>MHHHHHHMELSLASITVPLESIKPSNILPVTVYDQHGFRILFHFARDPLPGRSDVLVVVVSMLSTAPQPIRNIVFQSAVPKVMKVKLQPPSGMELPAFNPIVHPSAITQVLLLANPQKEKVRLRYKLTF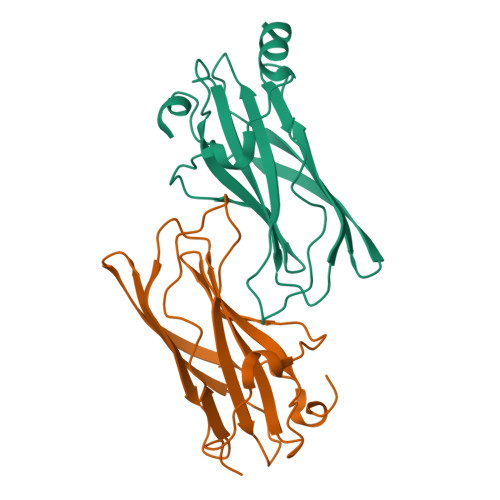TMGDQTYNEMGDVDQFPPPETWGSL[2x]>[2x]GSAMGSTVSVSKPLLKLKLLDCLRQSNFQQLCHLIANEFQPFDEPTVRSVFELILHYAVQVSPASLIKDIVQNWTTKGSSNSQLFIDVNKQDQDGNTPLHLAAFQSRGDVVTVLMNHPDINDCILNDAHLQPIEMCKNLNIAQMMQVARANYVAEIAQEFRQAFNNRDIDHLNSILSNPRNQELLDING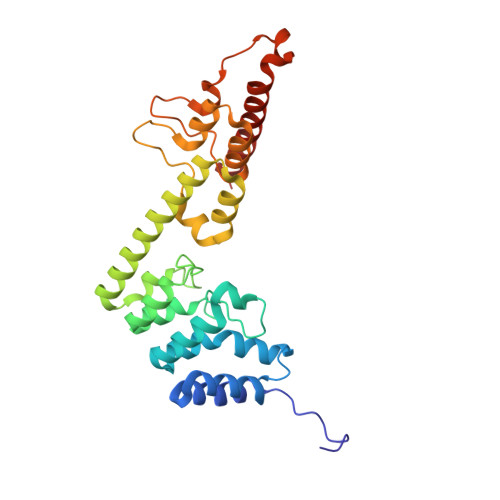MEPETGDTVLHEFVKKRDILLCRWILDHGGDPFKRDSRGKLPIDLLKKVSSKEQNDKKNAIDLELKKMLEKAAREQSVIDVT>SNATFLELVEVPCNSVHVQGVMTPNQMVKVTGAGWDNGVLEFYVTRPTKTGGDTSRSHLASIMCYSKDIDGVPSDKAGKCFLKRFSGEDSSEIDEKEVSLPIKSHNDAFMFVCSSNDGSALQCDVFALDNTNSNDGWKVNTVDLGVSVSPDLAFGLTADGVKVKKLYASSGLTAINDDPSLGCKA[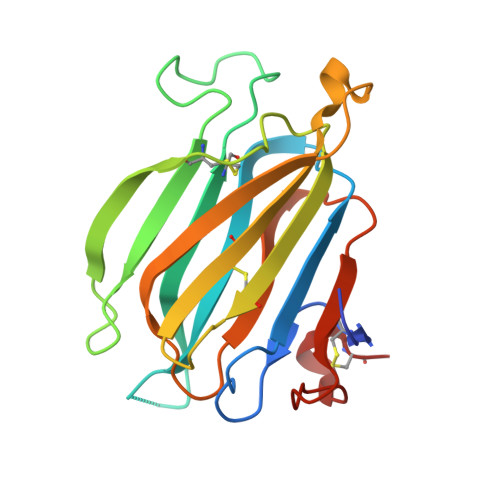3x]>[7x]SEEPSTVIMREAARHGLTIVRLQPQGSRLSLTVQPADFQALMAWLDALGQAGMT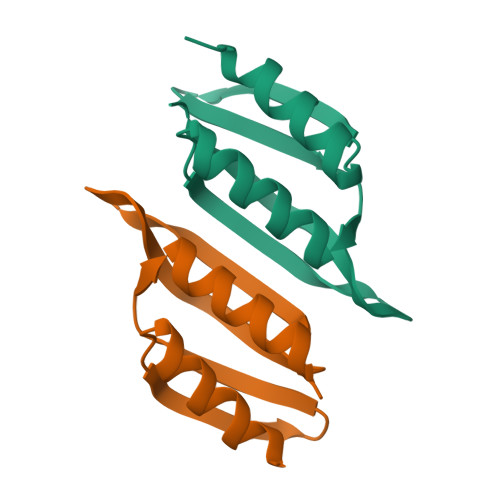TATLAVTAVAQQPGWVTVNTLVLERS The CDF transporter MamM is a highly conserved protein within magnetotactic bacteria (MTB). MTB are an extraordinary group of prokaryotes that utilize CDF proteins for iron transport and biomineralization of magnetic iron nanoparticles within intracellular membrane-enclosed organelles called magnetosomes. MamM was recently proposed to function as a magnetosome-directed iron transporter required for iron biomineralization, since its deletion abolished magnetite biomineralization. As a case study, we introduced ZnT-8 Type-II diabetes-associated mutations into the magnetosomal CDF protein MamM.

The X-ray determined structure of MamM-CTD V260R contained two tightly packed monomers in the asymmetric unit. Overlapping the monomers of wild-type MamM-CTD and the V260R mutant demonstrated that both share a similar fold, with a Cα-RMSD of 0.43 Å. While the wild-type MamM-CTD structure contains a disordered C-terminal tail (residues 293-318), a rigid conformation was adopted by residues 294-302 in a single V260R monomer comprising the dimer. This rigid C-terminal extension gave rise to the formation of a fourth β-sheet aligned in parallel to the three existing β-sheets located in the inner metal-binding interface of the dimer. The V260R dimer presented a tighter and twisted conformation in reference to wild-type MamM-CTD dimeric structure. As such, the V260R dimer structure presents a dramatic increase in the dimerization interface surface (377 Å2), in reference to the dimerization interface surface of the wild-type (193 Å2). According to the V260R determined structure, the altered dimerization interface is stabilized asymmetrically by several salt bridges, polar and hydrophobic interactions located at the top and bottom of the dimer. The twisted dimeric fold of V260R allows the formation of the central putative binding site but prevents the formation of the wild-type His264-Glu289 double peripheral binding sites. However, by examining the V260R dimer, we could predict two alternative peripheral symmetrical binding sites between Glu268-His264, each from a different monomer. Although the V260R mutant dimer was able to bind the same number of zinc cations as the wild-type dimer in vitro, it was not functional in vivo.

>[2x]GSHMEAVQNRIVEAAERVPGVRGVIHLRARYVGQDIWADMIIGVDPENTREQAHEICEAVQAAVCGKIRRIESLHVSAEAREIGDTTKPSFSDQPLSFDEVMLSKVDN> MAKSDVKLLGAWPSPYVMRARITLNVKSVDYELLEETLGSKSDLLLKSNPVHKKIPVLIHNDKPICESLIIVHYIDEFWSSGPSILPSDPYDRAIARFWAAYLDEKWYPSLKGIASAQGEEAKKAAVDQVGESLALIEDTYVKLSKGKPFF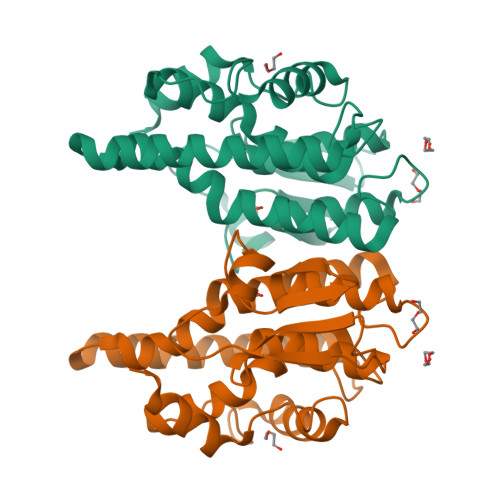GGEKIGYLDIAFGCFLGWLRVTEKTSGVKFLNEAKTPHLAKWAVRFCADPAVKDVMPETEKLAEFAKLLAKFRAGPPK>[4x]MNELVDTTEMYLRTIYDLEEEGVTPLRARIAERLDQSGPTVSQTVSRMERDGLLRVAGDRHLELTEK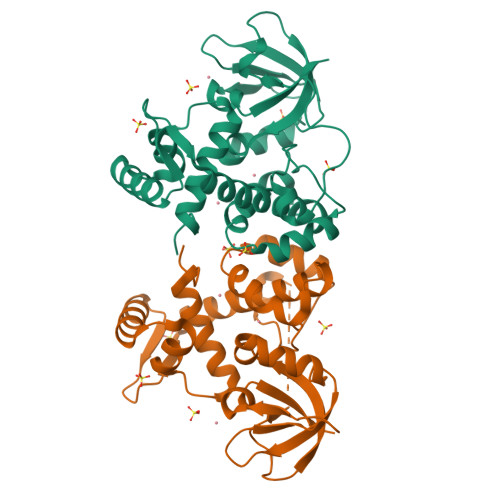GRALAIAVMRKHRLAERLLVDVIGLPWEEVHAEACRWEHVMSEDVERRLVKVLNNPTTSPFGNPIPGLDELGVGPEPGADDANLVRLTELPAGSPVAVVVRQLTEHVQGDIDLITRLKDAGVVPNARVTVETTPGGGVTIVIPGHENVTLPHEMAHAVKVEKV> MTKVTVVTGASRGLGEAIVKQILARNADAKVVAVARSAENLQKLEKGSEGRVLAVAGDVTRPETIHRLIEETVAKFGRIDSVVVNAGVLEPVQHIDSLDVDLVRRLYEVNLFSVMDLVRQTLPYMRQSKGSYLFVSSGASTKPYDAWSAYGSSKAALNYFCLSLATEEPLIRALSIAPGVVDTDMQQDIREVFGQNMAPDALKRFTDLHENKQLLAPEVPGGFYA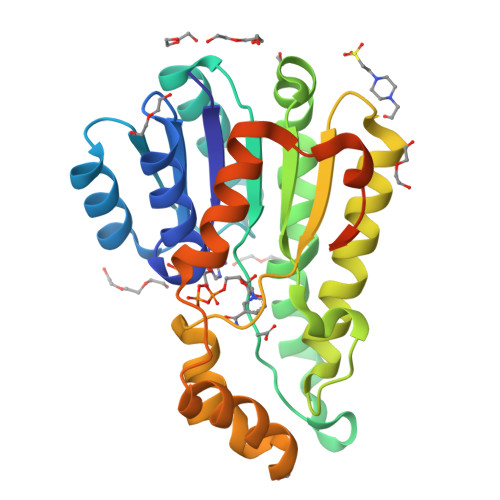SLALRGVPENLNGRYVRYDDSELKEYAKLAAALEHHHHHH> VSKLWVPNTDFDVAANWSQNRTPCAGGAVEFPADKMVSVLVQEGHAVSDMLLPLDGELVLASGAGFGVSDVGSHLDCGAGEPAVFRDSDRFSWHDPHLWRSGDEAPGLFFVDAERVPCRHDDVFFPPSASFRVGLGPGASPVRVRSISALGRTFTRDEDLAVFLASRAGRLRFHGPGALSVGPEDCADPSGCVCGNAEAQPWICAALLQPLGGRCPQAACHSALRPQGQCCDLCGAVVLLTHGPAFDLERYRARILDTFLGLPQYHGLQVAVSKVPRSSRLREADTEIQVVLVENGPETGGAGRLARALLADVAENGEALGVLEATMRESGAHVWGSS;>GELELQRQKRSINLQQPRMATERGNLVFLTGSAQNIEFRTGSLGKIKLNDEDLSECLHQIQKNKEDIIELKGSAIGLPQNISSQIYQLNSKLVDLERKFQGLQQTVDKKV[3x]

The intestinal uptake of B12 is a complex process that requires binding to the carrier protein ‘intrinsic factor’ (IF) and uptake of IF-B12 by the intestinal cubam receptor. Cubilin has been suggested to form trimers, which are anchored to the apical membrane via interaction with the type-1 transmembrane protein amnionless (AMN). AMN is formed by an extracellular domain, a transmembrane helix and a short cytoplasmic domain harbouring two adaptor protein-2-binding signals (Phe-X-Asn-Pro-X-Phe) for ligand-independent internalisation in clathrin-coated pits. As cubilin and AMN depend on each other for proper processing and translocation to the apical membrane, disrupted interaction of the two proteins leads to retention of both in the endoplasmic reticulum (ER).

For structural analysis, the ectodomain of AMN (20–357) and an N-terminal fragment of cubilin (26–135) were co-expressed in Escherichia coli. Crystals of the AMN(20–357)–cubilin(26–135) complex were obtained and the structure determined to 2.3 Å resolution by the single anomalous diffraction method. Electron density is observed for the entire ectodomain of AMN and for cubilin residues 37–120. The structure reveals a receptor architecture, where three cubilin chains combine into an intertwined β-helical structure that docks on to a corresponding β-helix domain in AMN. AMN forms a bean-shaped structure protruding ~60 Å from the plasma membrane and is composed of four structural entities. The fold of the two N-terminal domains of AMN (denoted β-helix 1 and β-helix 2) is similar and is formed by right-handed β-helices with hydrophobic cores. The head is formed by a three-turn intertwined β-helix, which irreversibly interlocks three cubilin chains. In the C-terminal region three cubilin chains form a coiled-coil, which is interrupted midway owing to the presence of a proline residue (Pro103). The cubilin interface with AMN is formed by the N-terminal strands of three cubilin chains (residues 42–49), which combine into a triangular face with a hydrophobic centre formed by Met44.> GAMALIEVEKPLYGVEVFVGETAHFEIELSEPDVHGQWKLKGQPLAASPDCEIIEDGKKHILILHNCQLGMTGEVSFQAAN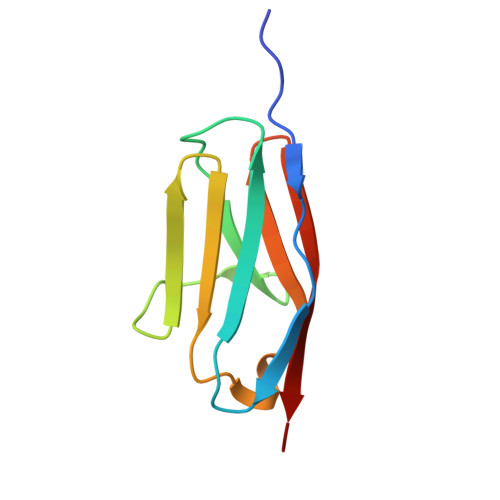TKSAANLKVKEL>MHHHHHHLEVLFQGPHMDEVIVNNISYHVGDWALLRNQNDPQKPIVGQIFRLW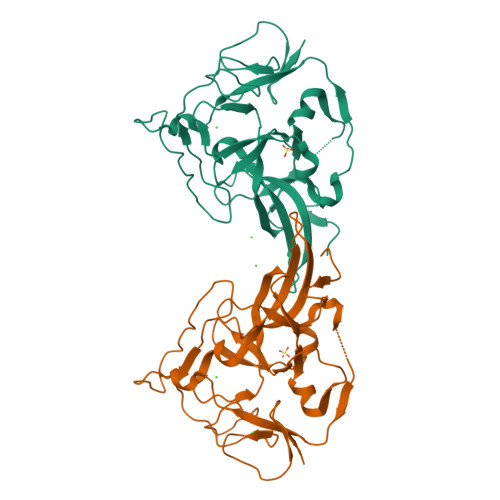KTPDGKQWLNACWYYRPEQTVHRVDRLFYKNEVMKTGQYRDHLVSNLVGKCYVIHFTRYQRGNPDMKLEGPLFVCEFRYNESDKIFNKIRTWKACLPEEIRDLDEATIPVNGRKFFKYPSPIRHLLPANATPHDRVPEPTMGSPDAPPLVGAVYMRPKMQRDDLGEYATSDDCPRYIIRPNDSPEEGQVDIETGTITTNTPTANA[4x]GcoA belongs to the CYP255A family of cytochrome P450 enzymes. Our recent characterization of a two-component P450 enzyme system consisting of a reductase, GcoB, and a P450 oxidase, GcoA, demonstrated that it demethylates diverse aromatic compounds, including guaiacol (which can be derived from coniferyl alcohol and represents the aromatic functionality of G-lignin that must undergo demethylation), guaethol, anisole (methoxybenzene), 2-methylanisole, and 3-methoxycatechol (3MC) with similar or greater efficiency than other O-aryl-demethylases described in the literature. However, GcoAB shows poor reactivity toward syringol, which can be derived from sinapyl alcohol via high-temperature reactions and represents the aromatic functionality of S-lignin that must undergo O-demethylation for further catabolism via ring-opening dioxygenases. In the present study, we hypothesized that substitution of GcoA-F169, which has the closest interaction with the bound substrate, may relax the specificity of the enzyme sufficiently to permit the O-demethylation of S-lignin type substrates.

The closest contact is with GcoA-F169, which forms a hydrophobic interaction with the C6 carbon on the aromatic ring of guaiacol. A broader survey of variants at the GcoA-F169 position (amino acids S, H, V, I, and L in addition to A) confirmed that GcoA-F169A exhibits the best catalytic performance in terms of both specific activity and reaction coupling, although other small side chains (S and V) also permitted reactivity with syringol, suggesting that these may permit syringol to assume a reactive conformation at the heme. Each protein variant also crystallized successfully with guaiacol and the structures showed that the orientation of the bound ligand remained consistent with that of the WT enzyme. Furthermore, comparison of the surrounding active site architecture confirmed no significant deviation from the WT.

> MTTTERPDLAWLDEVTMTQLERNPYEVYERLRAEAPLAFVPVLGSYVASTAEVCREVATSPDFEAVITPAGGRTFGHPAIIGVNGDIHADLRSMVEPALQPAEVDRWIDDLVRPIARRYLERFENDGHAELVAQYCEPVSVRSLGDLLGLQEVDSDKLREWFAKLNRSVTNAAVDENGEFANPEGFAEGDQAKAEIRAVVDPLIDKWIEHPDDSAISHWLHDGMPPGQTRDREYIYPTIYVYLLGAMQEPGHGMASTLVGLFSRPEQLEEVVDDPTLIPRAIAEGLRWTSPIWSATARISTKPVTIAGVDLPAGTPVMLSYGSANHDTGKYEAPSQYDLHRPPLPHLAFGAGNHACAGIYFANHVMRIALEELFEAIPNLERDTREGVEFWGWGFRGPTSLHVTWEV>[2x]GSHGMSKSPEEEHPVKAFGWAARDQSGHLSPFNFSRRATGEEDVRFKVLYCGVCHSDLHSIKNDWGFSMYPLVPGHEIVGEVTEVGSKVKKVNVGDKVGVGCLVGACHSCE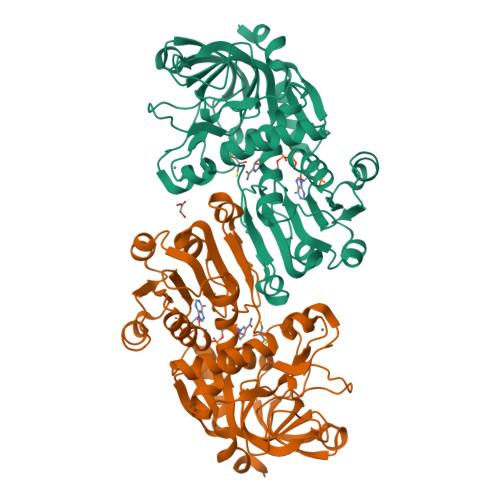SCANDLENYCPKMILTYASIYHDGTITYGGYSNHMVANERYIIRFPDNMPLDGGAPLLCAGITVYSPLKYFGLDEPGKHIGIVGLGGLGHVAVKFAKAFGSKVTVISTSPSKKEEALKNFGADSFLVSRDQEQMQAAAGTLDGIIDTVSAVHPLLPLFGLLKSHGKLILVGAPEKPLELPAFSLIAGRKIVAGSGIGGMKETQEMIDFAAKHNITADIEVISTDYLNTAMERLAKNDVRYRFVIDVGNTLAATKP> GAASMEFPFDVDALFPERITVLDQHLRPPARRPGTTTPARVDLQQQ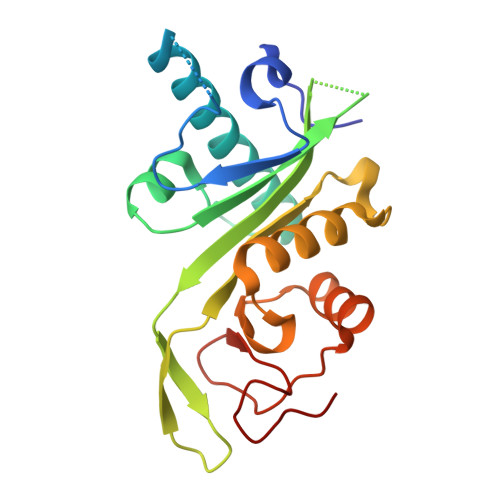IMTIIDELGKASAKAANLSAPITSASRMQSNRHVVYILKDSSARPAGKAAIIGFIKVGYKKLFVLDDREAHNEVEPLCILDFYIHESVQRHGHGRELFQYMLQKERVEPHQLAIDRPSQKLLKFLNKHYNLETTVPQVNNFVIFEGFFAHQHRP> RTEDLPKAVVFLEPQWYRVLEKDSVTLKCQGAYSPEDNSTQWFHNESLISSQASSYFID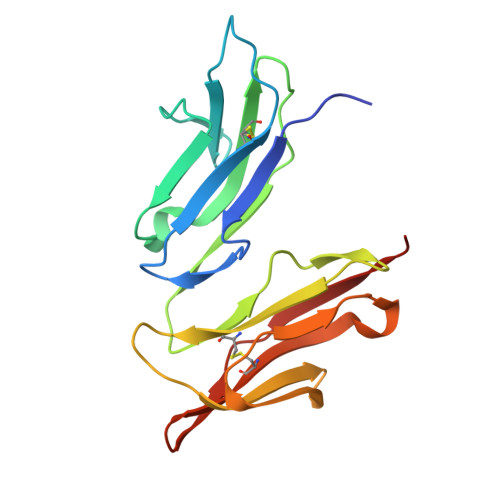AATVDDSGEYRCQTNLSTLSDPVQLEVHIGWLLLQAPRWVFKEEDPIHLRCHSWKNTALHKVTYLQNGKGRKYFHHNSDFYIPKATLKDSGSYFCRGLFGSKNVSSETVNITITQG> ARSTNTFNYATYHTLDEIYDFMDLLVAEHPQLVSKLQIGRSYEGRPIYVLKFSTGGSNRPAIWIDLGIHSREWITQATGVWFAKKFTEDYGQDPSFTAILDSMDIFLEIVTNPDGFAFTHSQNRLWRKTRSVTSSSLCVGVDANRNWDAGFGKAGASSSPCS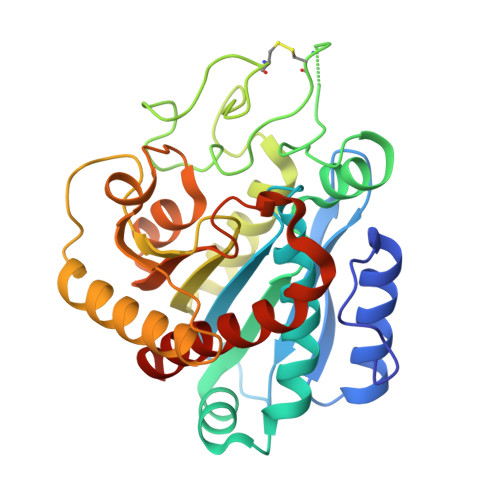ETYHGKYANSEVEVKSIVDFVKDHGNFKAFLSIHSYSQLLLYPYGYTTQSIPDKTELNQVAKSAVAALKSLYGTSYKYGSIITTIYQASGGSIDWSYNQGIKYSFTFELRDTGRYGFLLPASQIIPTAQETWLGVLTIMEHTVNNLY>VILTGNSSLCPI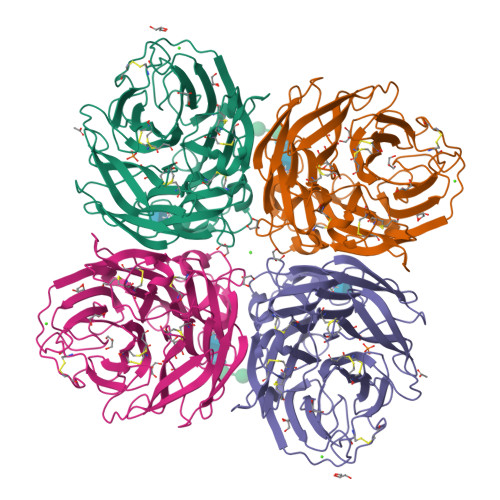SGWAIYSKDNGIRIGSKGDVFVIREPFISCSHLECRTFFLTQGALLNDKHSNGTVKDRSPYRTLMSCPVGEAPSPYNSRFESVAWSASACHDGMGWLTIGISGPDNGAVAVLKYNGIITDTIKSWRNNILRTQESECACVNGSCFTIMTDGPSNGQASYKILKIEKGKVTKSIELNAPNYHYEECSCYPDTGKVMCVCRDNWHGSNRPWVSFDQNLDYQIGYICSGVFGDNPRPNDGTGSCGPVSSNGANGIKGFSFRYDNGVWIGRTKSTSSRSGFEMIWDPNGWTETDSSFSVRQDIVAITDWSGYSGSFVQHPELTGLDCMRPCFWVELIRGQPKENTIWTSGSSISFCGVNSDTVGWSWPDGAELPFSIDK[2x]>MQSTPLLQIQPHFHVEVIEPKQVYLLGEQANHALTGQLYCQILPLLNGQYTLEQIVEKLDGEVPPEYIDYVLERLAEKGYLTEAAPELSSEVAAFWSELGIAPPVAAEALRQPVTLTPVGNISEVTVAALTTALRDIGISVQTPTEAGSPTALNVVLTDDYLQPELAKINKQALESQQTWLLVKPVGSVLWLGPVFVPGKTGCWDCLAHRLRGNREVEASVLRQKQAQQQRNGQSGSVIGCLPTARATLPSTLQTGLQFAATEIAKWIVKYHVNATAPGTVFFPTLDGKIITLNHSILDLKSHILIKRSQCPTCGDPKILQHRGFEPLKLESRPKQFTSDGGHRGTTPEQTVQKYQHLISPVTGVVTELVRITDPANPLVHTYRAGHSFGSATSLRGLRNTLKHKSSGKGKTDSQSKASGLCEAVERYSGIFQGDEPRKRATLAELGDLAIHPEQCLCFSDGQYANRETLNEQATVAHDWIPQRFDASQAIEWTPVWSLTEQTHKYLPTALCYYHYPLPPEHRFARGDSNGNAAGNTLEEAILQGFME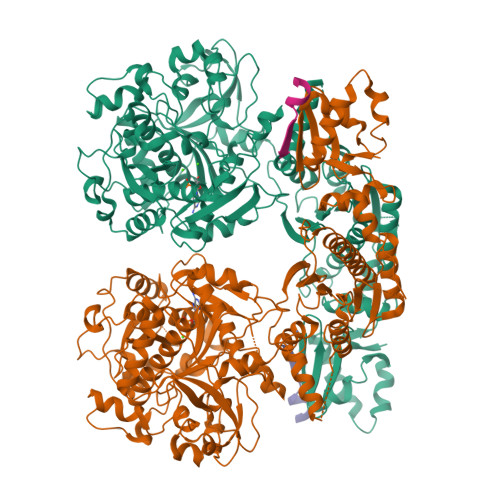LVERDGVALWWYNRLRRPAVDLGSFNEPYFVQLQQFYRENDRDLWVLDLTADLGIPAFAGVSNRKTGSSERLILGFGAHLDPTIAILRAVTEVNQIGLELDKVPDENLKSDATDWLITEKLADHPYLLPDTTQPLKTAQDYPKRWSDDIYTDVMTCVNIAQQAGLETLVIDQTRPDIGLNVVKVTVPGMRHFWSRFGEGRLYDVPVKLGWLDEPLTEAQMNPTPMPF[2x];>[2x]MDKKNILPQQGQPVIRLTAGQLSSQLAELSEEALGDAGLEASKITACITFCAYDGELEHHHHHH> QIYTIIEELCIGCGFCTDECPP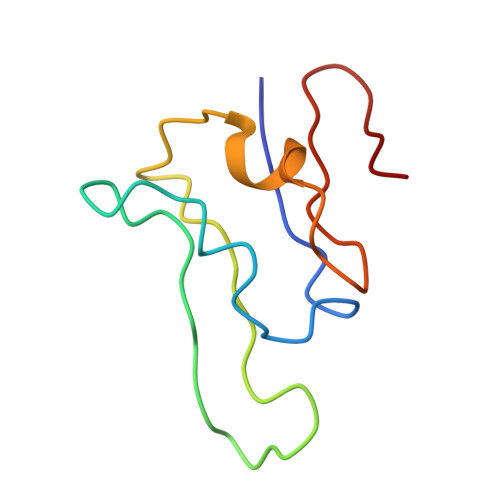KVNAILPRDVEAVLDGGETYWIDQTRCISCSLCFVAGTCPTDAVVFTEGGVSRT>[4x]MRILFIGDVVGSPGRDMVKEYVPKLKTKYKPHFTIINGENAAHGKGLTEKIYHSLIQSGADAITMGNHTWDKKEIFDFIDDV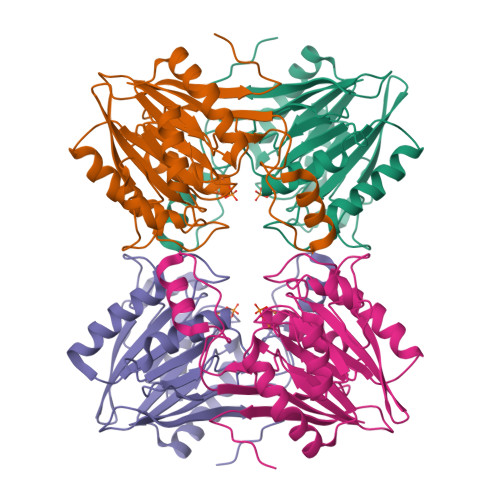PNLVRPANFPEGTPGKGITYVKANGKELAVINLQGRTFLPPLDDPFLKADELIAEAAKRTPYIFIDFHAEATSEKLALGWYTDGRASAVVGTHTHVQTADNRILPKGTAYITDVGMTGPYDGILGMDRETIIKRFKTNLPVRFTVAEGKTTLSGVVIDIDDQTKKAVKIERILINDDHMFFELDPNSSSVDKLAAALEHHHHHH>[4x]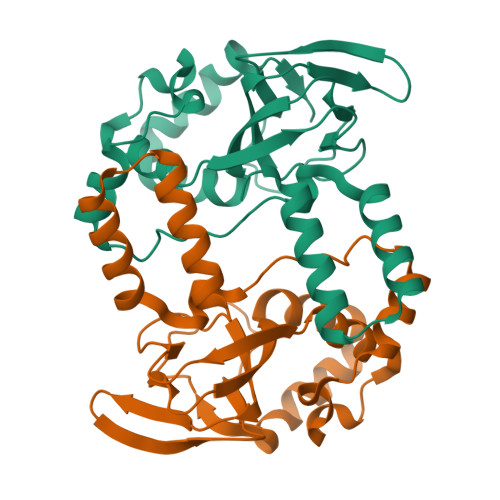GAMDQRMYSRRSLYHTRTKDLKDFIRVHRLPKALAQRMLECFQTTWSVNNGIDVSELLKDFPDELRADIAMHLNKELLQLPLFESASRGCLRSLSLIIKTSFCAPGEFLIRQGDALQAIYFVCSGSMEVLKDNTVLAILGKGDLIGSDSLTKEQVIKTNANVKALTYCDLQYISLKGLREVLRLYPEYAQKFVSEIQHDLTYNLREGSGADL>GVVTSE[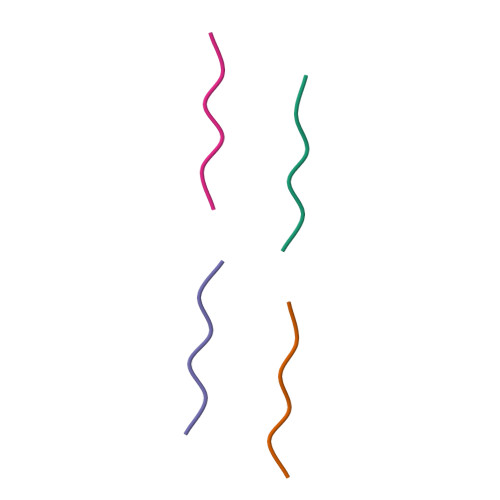4x]> GDLKTAVFNAARDGKLRLLTKLLASKSKEEVSSLISEKTNGATPLLMAARYGHLDMVEFLLEQCSASIEVGGSVNFDGETIEGAPPLWAASAAGHLKVVQSLLNHGASVNNTTLTNSTPLRAACFDGHLEIVKYLVEHKADLEVSNRHGHTCLMISCYKGHKEIAQYLLEKGADVNRKSVKGNTALHDCAESGSLDIMKMLLMYCAKMEKDGYGMTPLLSASVTGHTNIVDFLTHHAQTSKTERINALELLGATFVDKKRDLLGALKYWKKAMNMRYSDRTNIISKPVPQTLIMAYDYAKEVNSAEELEGLIADPDEMRMQALLIRERILGPSHPDTSYYIRYRGAVYADSGNFKRCINLW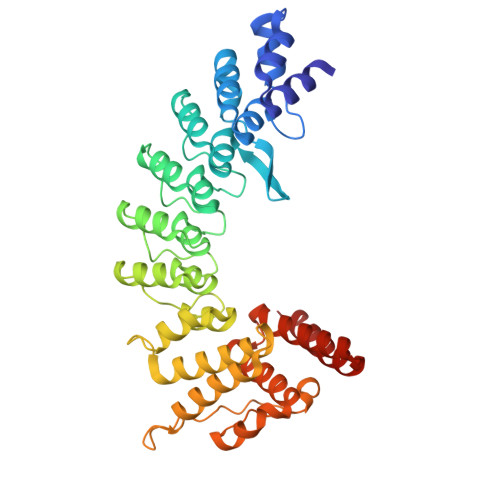KYALDMQQSN> GGACAGA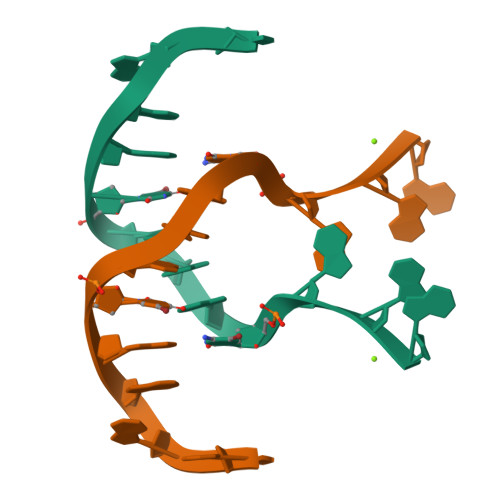UGGGAG> MSNISRQAYADMFGPTVGDKVRLADTELWIEVEDDLTTYGEEVKFGGGKVIRDGMGQGQMLAADCVDLVLTNALIVDHWGIVKADIGVKDGRIFAIGKAGNPDIQPNVTIPIGAATEVIAAEGKIVTAGGIDTHIHWICPQQAEEALVSGVTTMVGGGTGPAAGTHATTCTPGPWYISRMLQAADSLPVNIGLLGKGNVSQPDALREQVAAGVIGLKIHEDWGATPAAIDCALTVADEMDIQVALHSDTLNESGFVEDTLAAIGGRTIHTFHTEGAGGGHAPDIITACAHPNILP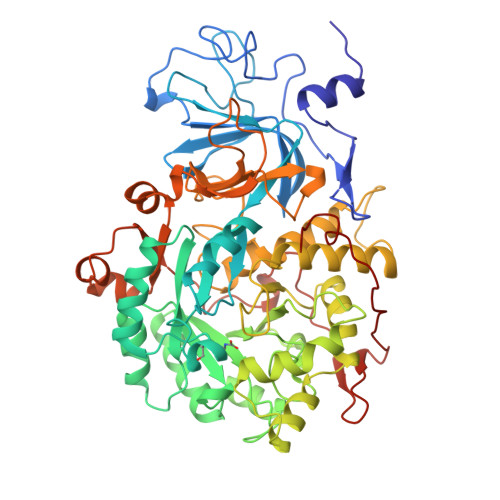SSTNPTLPYTLNTIDEHLDMLMVSHHLDPDIAEDVAFAESRIRRETIAAEDVLHDLGAFSLTSSDSQAMGRVGEVILRTWQVAHRMKVQRGALAEETGDNDNFRVKRYIAKYTINPALTHGIAHEVGSIEVGKLADLVVWSPAFFGVKPATVIKGGMIAIAPMGDINASIPTPQPVHYRPMFGALGSARHHCRLTFLSQAAAANGVAERLNLRSAIAVVKGCRTVQKADMVHNSLQPNITVDAQTYEVRVDGELITSEPADVLPMAQRYFLF>[6x]KEENNFINLYTVKNPLKCKIVDKINLVRPNSPNEVYHLEINHNGLFKYLEGHTCGIIPYYNELDNNPNNQINKDHNIINTTNHTNHNNIALSHIKK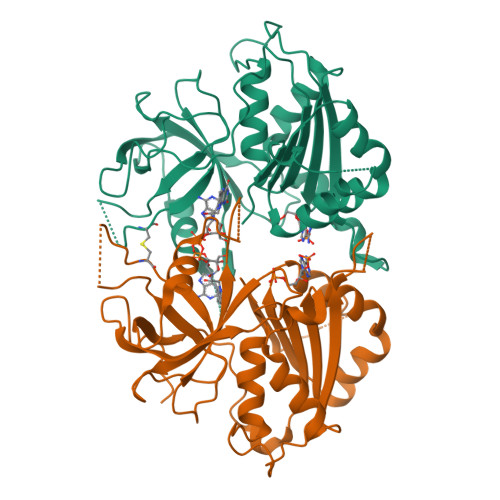QRCARLYSISSSNNMENLSVAIKIHKYEQTENAPNITNYGYCSGFIKNLKINDDIYLTGAHGYFNLPNDAIQKNTNFIFIATGTGISPYISFLKKLFAYDKNNLYNRNSNYTGYITIYYGVYNEDSILYLNELEYFQKMYPNNINIHYVFSYKQNSDATSFYVQDEIYKRKTEFLNLFNNYKCELYICGLKSIRYKVMDILKSHDQFDEKKKKRVHVEVY> QDTSPDTLVVTANRFEQPRSTVLAPTTVVTRQDIDRWQSTSVNDVLRRLPGVDITQNGGSGQLSSIFIRGTNASHVLVLIDGVRLNLAGVSGSADLSQFPIALVQRVEYIRGPRSAVYGSDAIGGVVNIITTRDEPGTEISAGWGSNSYQNYDVSTQQQLGDKTRVTLLGDYAHTHGYDVVAYGNTGTQAQTDNDGFLSKTLYGALEHNFTDAWSGFVRGYGYDNRTNYDAYYSPGSPLLDTRKLYSQSWDAGLRYNGELIKSQLITSYSHSKDYNYDPHYGRYDSSATLDEMKQYTVQWANNVIVGHGSIGAGVDWQKQTTTPGTGYVEDGYDQRNTGIYLTGLQQVGDFTFEGAARSDDNSQFGRHGTWQTSAGWEFIEGYRFIASYGTSYKAPNLGQLYGFY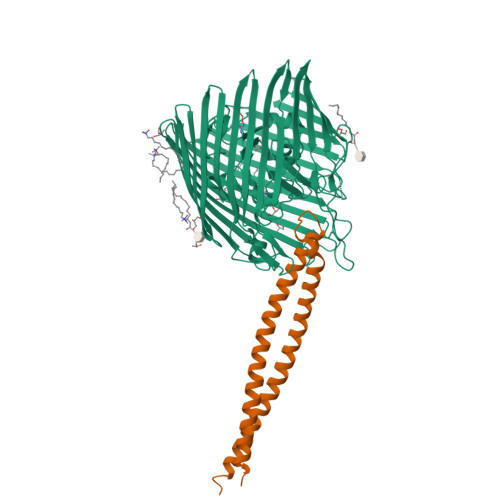GNPNLDPEKSKQWEGAFEGLTAGVNWRISGYRNDVSDLIDYDDHTLKYYNEGKARIKGVEATANFDTGPLTHTVSYDYVDARNAITDTPLLRRAKQQVKYQLDWQLYDFDWGITYQYLGTRYDKDYSSYPYQTVKMGGVSLWDLAVAYPVTSHLTVRGKIANLFDKDYETVYGYQTAGREYTLSGSYTF;> HPVEAAERNYERARAELNQANEDVARNQERQAKAVQVYNSRKSELDAANKTLADAIAEIKQFNRFAHDPMAGGHRMWQMAGLKAQRAQTDVNNKQAAFDAAAKEKSDADAALSSAMESRKKKEDKKRSAENNLND>MGNTKKTTDSSAGVLATVDGRPITKSDFDMIKQRNPNFDFDKLKEKEKEALIDQAIRTALVENEAKTEKLDSTPEFKAMMEAVKKQALVEFWAKKQAEEVKKVQIPEKEMQDFYNANKDQLFVKQEAHARHILVKTEDEAKRIISEIDKQPKAKKEAKFIELANRDTIDPNSKNAQNGGDLGKFQKNQMAPDFSKAAFALTPGDYTKTPVKTEFGYHIIYLISKDSPVTYTYEQAKPTIKGMLQ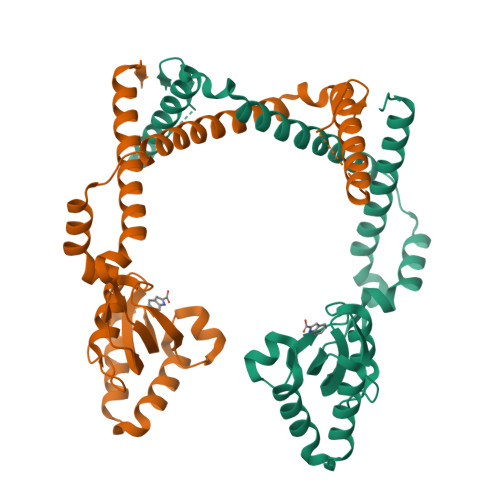EKLFQERMNQRIEELRKHAKIVINKLEHHHHHH[2x]>[2x]MNTVDVNMMDNNPAARLEELRTIMKKNKIDVYILINSDEHNSEIIN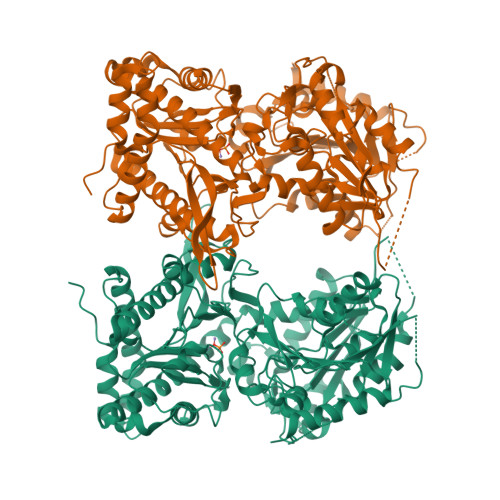EKDKKIVKITNYSGADGILIVTKDKPILYVNALYELQAMNELDQNLFTLRISRIDNRDEIFETISSLEFNTIAFDGKNTSVVFYEKLRKALLNAYPKKKIVEKIIYNNNFDDVNKKDDENVLNFLVLEKSLVEIKDYPVNNKTLYIHDRKYNGACAGEKIDKLKQSLMYDIKNVDNLLLSELDEIAYLLNLRGYDYQYSPLFYSYLLFQFDREEQDFSKIVFFTTVKNLPADVKNLLEINKVIVKEYEEIVPYLRDVVIPSIPKHNDDNPDFKKYDISLSPYINLMIYKLFDRKNVLLQNSPVVKMKAVKNDVEIDNMKQAHILDGLALLQFFHWCEQKRKTKELFNETEMSLRHKVDYFRSTKKNFIFPSFSTISASGPNAAVIHYECTDKTNATIKPAIYLLDSGGQYLHGTTDVTRTTHFGEPTAEEKRIYTLVLKGHLRLRKVIFASYTNSSALDFIARENLFNNFMDYNHGTGHGVGLTLNVHEGGCSIGPVGGAPLKKNMVLSNEPGYYMKDKFGVRIENMQYVISKEITDTTEYLSFDDLTMYPYEKKLLDFSLLTNQEIKELNEYHTTIRNTLLPLVKQSPQEYGESVEKYLIEITEPIAIHNNHHHHHH>[6x]MANLERTFIAIKPDGVQRGLVGEIIKRFEQKGFRLVAMKFLRASEEHLKQHYIDLKDRPFFPGLVKYMNSGPV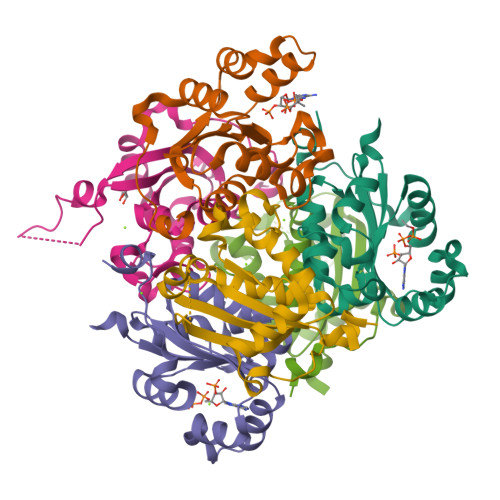VAMVWEGLNVVKTGRVMLGETNPADSKPGTIRGDFCIQVGRNIIHGSDSVKSAEKEISLWFKPEELVDYKSCAHDWVYE(4AS,8AR)-4-(3-{4-[(3R)-3-HYDROXYPYRROLIDINE-1- 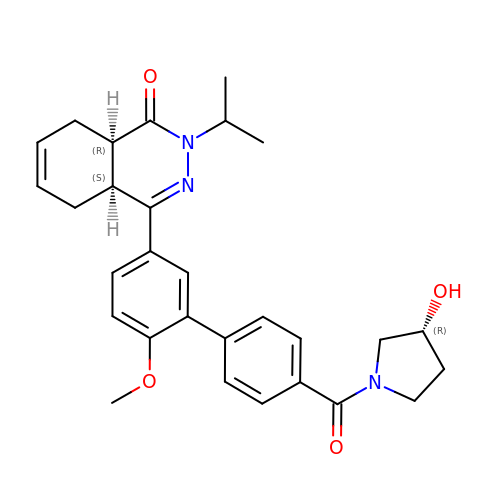| C29 H33 N3 O4 | UNEWFLJRNQWALM-TZRRMPRUSA-N>[4x]MAPVEFPKSLRASSHSSEGGTTKEEDIYGYELLYRSAFASYIAPTGAWNLV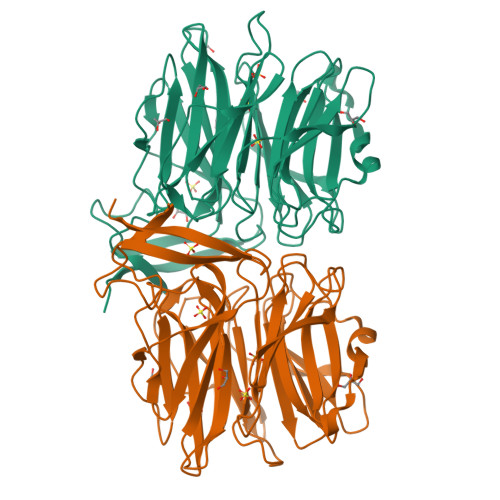WFQAADGSIKQARWYGEWVISTVLAPGKALQGTPLTALLWGPQDTVALYYLSPQFELQEWCWDTKNGADNKYDGALNAAKVKVAPYSKLGAVSFGGANLAVYYQGTNNKLEEYTFGGGQGWKKGATLPGDPLPGTYISFVNRNKWDANPPSIAGYFQTVTGSLAEQVWETGGWRIGQFVIPAAPFLTPISATVSPEKDFPKIHVYWLSVESTIIESVNWHGWKAPKQIDNISVVKADISATSFTRDDGTVDVRIYGTAQLNVLFERIFRYGVWEEKIHSISVGKEIPIEVVGVAAALEHHHHHH>UAGGGU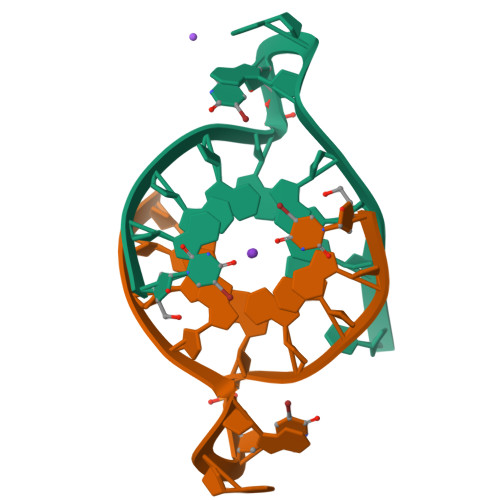TAGGGT[2x]> KNFKTDLIRMQWPAMRDEMVRFFQSQNAIAFDKISKRHPSASLSSDASSSSSSPSANRGERRATAEEVDREEQGKLSFAEMVVGSTRSACGVLGAGRSSAVDVACKPWKRFVRKEDIQRAGYVPCIVEKYGIERRLAIHRDTLEALAFDEQHGHLSYLFQARLFRLRIGNWIEECIPTF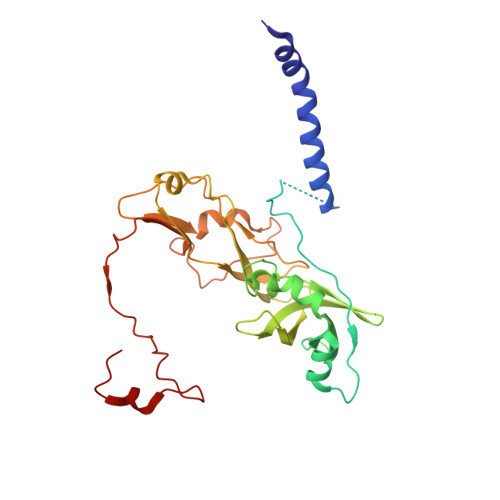VQADPVARRLYFVKFERHVAGKISEVDIPTTMVGLLACPAYQRGYHVELVMPTIRCQCVGAEIPPPFFVDVSRLHYSPPYTAITLQDLQHLLPADGSARFHPSYDAATQEVAWAYEVGSLPDAPLPADYVDPNFVDRKGQKMDVCFRNHFPN> GPMRSRIFKIIVIGDSNVGKTCLTYRFCAGRFPDRTEATIGVDFRERAVEIDGERIK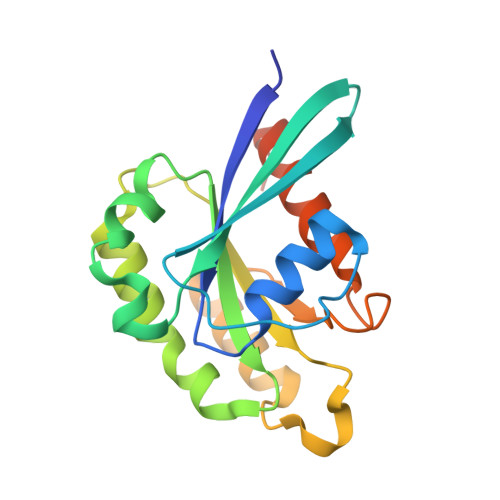IQLWDTAGQERFRKSMVQHYYRNVHAVVFVYDMTNMASFHSLPSWIEECKQHLLANDIPRILVGNKCDLRSAIQVPTDLAQKFADTHSMPLFETSAKNPNDNDHVEAIFMTLAHKLKSHKPLMLSQPPDNGIILK> DEQSG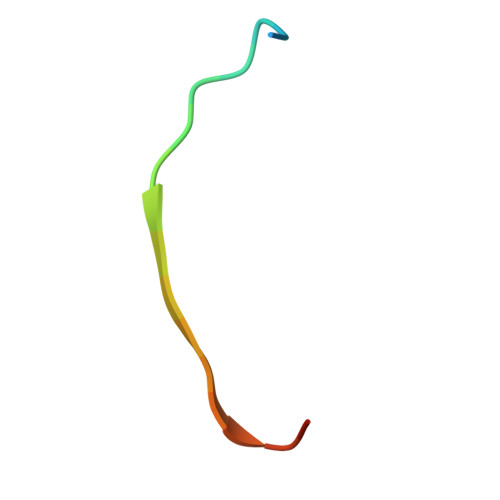ISQTVIVGPWGAKSA> GNSVTNIYGNGNNVTTDVGANGWAPTVSTGLGDGPVSASADSLPGRSGGASSEKTHTVSGSSNKVGSRFSKWWEPAAARASESATDSAIEGIDAAGKAASKAITRKLDRPAAPSSTANPQPSLIALNPSATQSGNASILTGSTAPSLLAYPTATPVPLPNPDEPSQPGPSGDRTWLLDTVTWSQEFTRG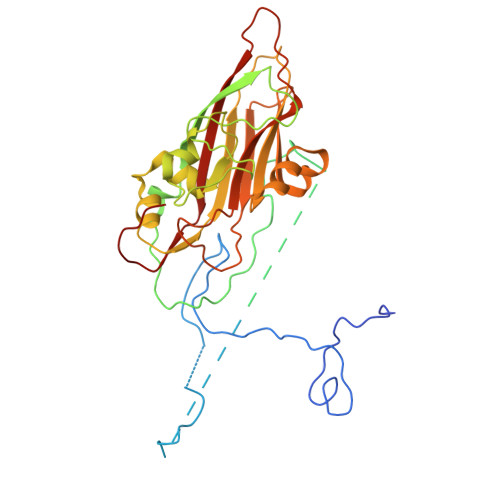WNIAGSNGMQWTGLESLIFPVSTDTNWTSTSSPTAYPLPFSFVRAYPDSSWAAMYNTHSMWNCGWRVQVTVNGSQFHAGALILYMVPEATTHAIQTARDNAGFVFPYVILNLYESNTATIEVPYISPTPNTSSGLHAPWTFYLQVLSPLNPPPSLPTSLSCSIYVTPVDSSFHGLRYLAPQ>ADYIEMKVPAQPEYVGIIRLTLSGVASRMGYTYDEIEDLKIAVSEACTNAVQHAYKEDKNGEVSIRFGVFEDRLEVIVADEGDSFDFDQKQQDLGPYTPSHTVDQLSEGGLGLYLMETLMDEVRVQNHSGVTVAMTKYLNG[8x];>[8x]NINVDVKQNENDIQVNIAGEIDVYSAPVLREKLVPLAEQGADLRICLKDVSYMDSTGLG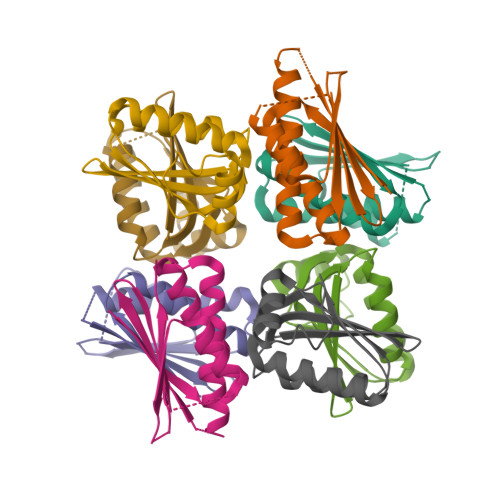VFVGTFKMVKKQGGSLKLENLSERLIRLFDITGLKDIIDISAKS> MKRRFTLLGSVVALALSSTALASDAPASRGCADDAGWNDPAMPLKVYGNTWYVGTCGISALLVTSDAGHILVDAATPQAGPQILANIRALGFRPEDVRAIVFSHEHFDHAGSLAELQKATGAPVYARAPAIDTLKRGLPDRTDPNFEVAEPVAPVANIVTLADDGVVSVGPLALTAVASPGHTPGGTSWTWRSCEGDDCRQMVYADSLTAISDDVFRYSDDAAHPGYLAAFRNTLARVAALDCDILVTPHPSASGLWNR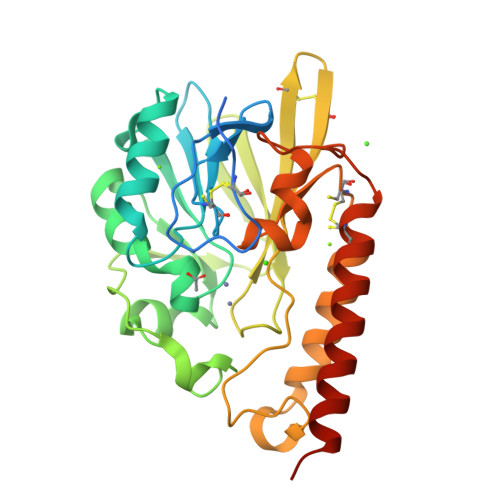IGPRAAAPLMDTTACRRYAQGARQRLEKRLAEEAATSPSSGARP> MSGDTTLVDTVNASQSRQVFWDRDVYDLEIERIFSRAWLMLGHKSLLPKPGDFITTYMAEDKIILSHQSDGTFRAFINSCTHRGNQICHADSGNAKAFVCNYHGW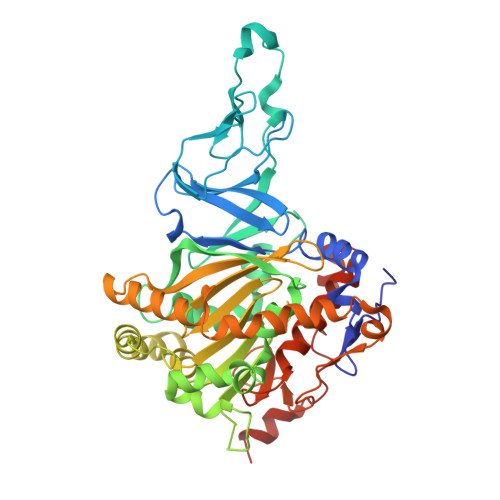VYGQDGSLVDVPLESRCYHNKLDKQELAAKSVRVETYKGFIFGCHDPEAPSLEDYLGEFRFYLDTIWEGGGAGLELLGPPMKSLLHCNWKVPVENFVGDGYHVGWTHAAALGQIGGPLAGLAGNRADIPFDDLGLQFTTRHGHGFGVIDNAAAAIHRKGDGWNKYLEDTRGEVRRKFGADRERLYVGHWNGAIFPNCSFLYGTNTFKIWHPRGPHEIEVWTYTMVPSDADPATKSAIQREATRTFGTAGTLESDDGENMSSATYVNRGVITRDGMMNSTMGVGYEGPHPVYPGIVGISFIGETSYRGFYRFWKEMIDAPDWASVKANDDNWDSVFTNRNFWNEKLNAAE> MKNRNRMIVNGIVTSLICCSSLSALAASPPTEVKIVRDEYGMPHIYADDTYRLFYGYGYVVAQDRLFQMEMARRSTQGTVSEVLGKAFVSFDKDIRQNYWPDSIRAQIASLSAEDKSILQGYADGMNAWIDKVNASPDKLLPQQFSTFGFKPKHWEPFDVAMIFVGTMANRFSDSTSEIDNLALLT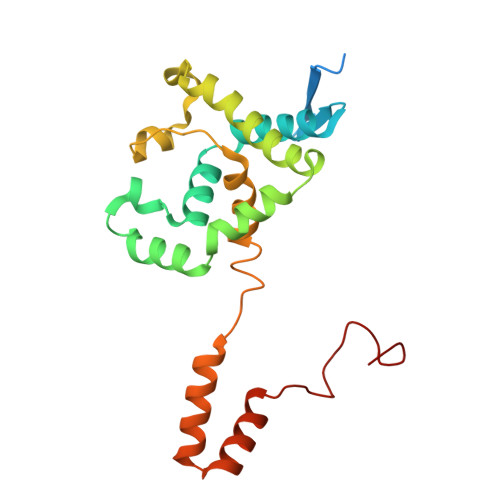ALKDKYGKQQGMAVFNQLKWLVNPSAPTTIAARESA> TEATAGTVTVNAITSDDTIDGIELGQTISISGKAVGGDISVGDVVKMTINNTEYSTTVKAGGIWMIAGVLGSDLAADSEFDVVVTSSDAAGNKVQSIGTSTHSVDLSAEANFSLAEGQQHVLTNLPEGFGFPDGTTEVVTNFGGTITLGDDGEYRYDAPVRDHGDAVSDKDSVTVTLEDGRTFTVNLDIQDSAPVAVDDQDSIVVQHEEFEVSEIAASWVSYTHGESVTTFDGTSDLGGVDNDSAKDQIRWGNPAESKQSGYGFIDNDSNLEGRFDLNQDISVGTFTHYNYPVYSGGAITSAEMSVEFSVLDHLGVSTPVTLTVNFDHNETPNTNDVNASRDIVTVQNTHVTFERDGDIYTVQIVGFREVGNPDGEVVTSIYTNENAATSYELVVRVVEGDGYSLPSTEGNIFDDNGLGADSL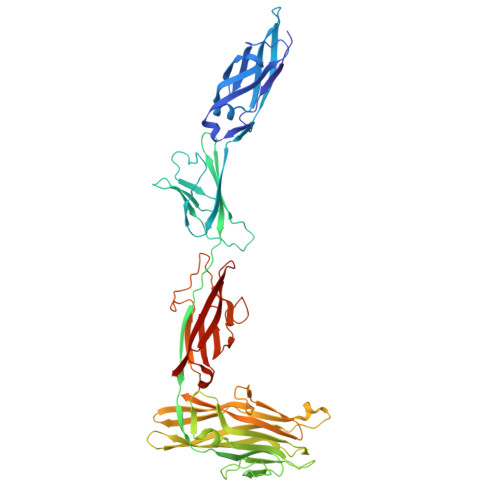GADGSVTVVGVAVGAIVSSNESVGHSIEGQYGNLVLNSDGSYVYDVTASVSDIPAGATESFAYLIQDQDGSTSSANLSINVGTN>[2x]GSGNSASQSPFSNPNTAEAFARSFVSNIVSSGEFGAQGAEDFDDIIQSLIQ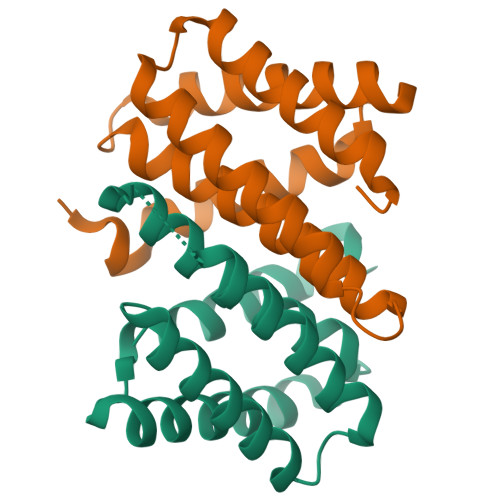AQSMGKGRHDTKAKAKAMQVALASSIAELVIAESSGGDVQRKTNVISNALRNALMSTTGSPNEEFVHEVQDLIQMLSQEQINEV> GPGLKQKIVIKVAMEGNNCRSKAMALVASTGGVDSVALVGDLRDKIEVVGYGIDPIKL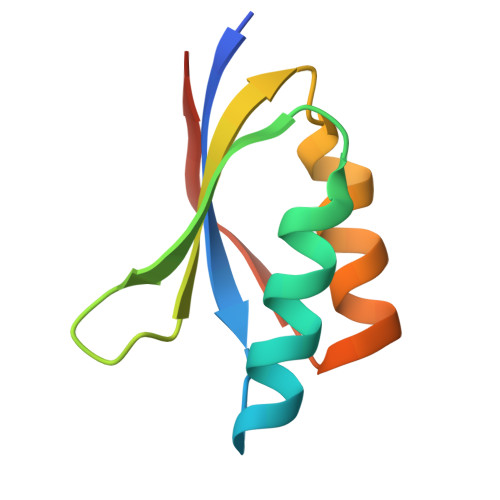ISALRKKVGDAELLQVEQAKED>[4x]MNTINIAKNDFSDIELAAIPFNTLADHYGERLAREQLALEHESYEMGEARFRKMFERQLKAGEVADNAAAKPLITTLLPKMIARINDWFEEVKAKRGKRPTAFQFLQEIKPEAVAYITIKTTLACLTSADNTTVQAVASAIGRAIEDEARFGRIRDLEAKHFKKNVEEQLNKRVGHVYKKAFMQVVEADMLSKGLLGGEAWSSWHKEDSIHVGVRCIEMLIESTGMVSLHRQNAGVVGQDSETIELAPEYAEAIATRAGALAGISPMFQPCVVPPKPWTGITGGGYWANGRRPLALVRTHSKKALMRYEDVYMPEVYKAINIAQNTAWKINKKVLAVANVITKWKHCPVEDIPAIEREELPMKPEDIDMNPEALTAWKRAAAAVYRKDKARKSRRISLEFMLEQANKFANHKAIWFPYNMDWRGRVYAVSMFNPQGNDMTKGLLTLAKGKPIGKEGYYWLKIHGANCAGVDKVPFPERIKFIEENHENIMACAKSPLENTWWAEQDSPFCFLAFCFEYAGVQHHGLSYNCSLPLAFDGSCSGIQHFSAMLRDEVGGRAVNLLPSETVQDIYGIVAKKVNEILQADAINGTDNEVVTVTDENTGEISEKVKLGTKALAGQWLAYGVTRSVTKRSVMTLAYGSKEFGFRQQVLEDTIQPAIDSGKGLMFTQPNQAAGYMAKLIWESVSVTVVAAVEAMNWLKSAAKLLAAEVKDKKTGEILRKRCAVHWVTPDGFPVWQEYKKPIQTRLNLMFLGQFRLQPTINTNKDSEIDAHKQESGIAPNFVHSQDGSHLRKTVVWAHEKYGIESFALIHDSFGTIPADAANLFKAVRETMVDTYESCDVLADFYDQFADQLHESQLDKMPALPAKGNLNLRDILESDFAFA

Bacteriophage T7 RNA polymerase (T7 RNAP) is widely used for synthesizing RNA molecules with synthetic modifications and unnatural base pairs (UBPs) for a variety of biotechnical and therapeutic applications. A 7-(2-thienyl)-imidazo[4,5-b]pyridine (Ds) and pyrrole 2-carbaldehyde (Pa) pair, developed by Hirao group, is a representative hydrophobic UBP that relies on shape complementarity and hydrophobic interactions, but lacks hydrogen bonding between the base pairs. Our kinetic assays revealed that T7 RNAP selectively recognizes the Ds or Pa base in the templates and preferentially incorporates their cognate unnatural base nucleotide substrate (PaTP or DsTP) over natural NTPs. To understand the structural basis of UBP transcription, we solved six T7 RNAP–UBP complex structures with or without its cognate substrates (dDs, dPa apo structures, dDs–PaTP, dPa–DsTP, dDs–ATP, dPa–ATP complex structures).

We crystallized T7 RNAP containing a site-specific dDs or dPa at the +1 position of the template strand DNA. The overall structures of UB-containing T7 RNAP elongation complexes are essentially identical to that of natural T7 RNAP. T7 RNAP is captured at the post-translocation state, where the elongation complex is waiting for incoming substrate and gating Y639 is stacking with the −1 template-strand base. Both dDs and dPa are accommodated at a binding pocket over the O-helix, essentially the same as the natural bases. Intriguingly, we observed UB-specific interactions between the unnatural base and T7 RNAP. The dDs base fits perfectly to the surface of the O-helix and appears to interact with R632 via hydrogen bonding between the sulfur atom in Ds and the carboxyl group in R632. First, in the post-translocation state (apo), the dDs or dPa template base can be easily loaded at the pocket above O-helix with similar conformation to that of natural bases.> GPLGSMPGEEEERAFLVAREELASALRRDSGQAFSLEQLRPLLASSLPLAARYLQLDAARLVRCNAHGEPRNYLNTLSTALNILEKYGRNLLSPQRPRYWRGVKFNNPVFRSTVDAVQGGRDVLRLYGYTEEQPDGLSFPEGQEEPDEHQVATVTLEVLLLRTELSLLLQNTHP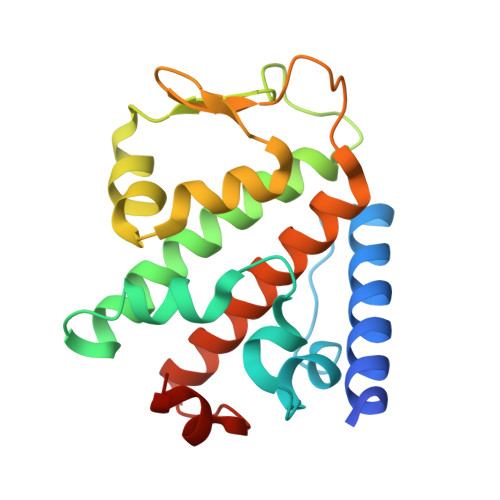RQQALEQLLE> TGLAADIRWTAYGVPHIRAKDERGLGYGIGYAYARDNACLLAEEIVTARGERARYFGSEGKSSAELDNLPSDIFYAWLNQPEALQAFWQAQTPAVRQLLEGYAAGFNRFLREADGKTTSCLGQPWLRAIATDDLLRLTRRLLVEGGVGQFADALVAAAPPGAEK;> SNAIAVGSERSADGKGMLLANPHFPWNGAMRFYQMHLTIPGRLDVMGASLPGLPVVNIGFSRHLAWTHTVDTSSHFTLYRLALDPKDPRRYLVDGRSLPLEEKSVAIEVRGADGKLSRVEHKVYQSIYGPLVVWPGKLDWNRSEAYALRDANLENTRVLQQWYSINQASDVADLRRRVEALQGIPWVNTLAADEQGNALYMNQSVVPYLKPEL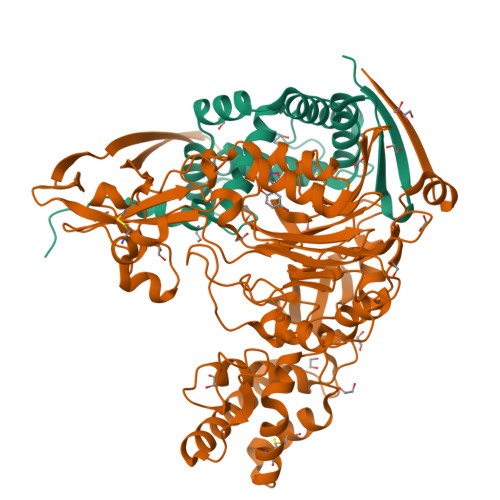IPACAIPQLVAEGLPALQGQDSRCAWSRDPAAAQAGITPAAQLPVLLRRDFVQNSNDSAWLTNPASPLQGFSPLVSQEKPIGPRARYALSRLQGKQPLEAKTLEEMVTANHVFSADQVLPDLLRLCRDNQGEKSLARACAALAQWDRGANLDSGSGFVYFQRFMQRFAELDGAWKEPFDAQRPLDTPQGIALDRPQVATQVRQALADAAAEVEKSGIPDGARWGDLQVSTRGQERIAIPGGDGHFGVYNAIQSVRKGDHLEVVGGTSYIQLVTFPEEGPKARGLLAFSQSSDPRSPHYRDQTELFSRQQWQTLPFSDRQIDADPQLQRLSIRE3-PHENYLPYRUVIC 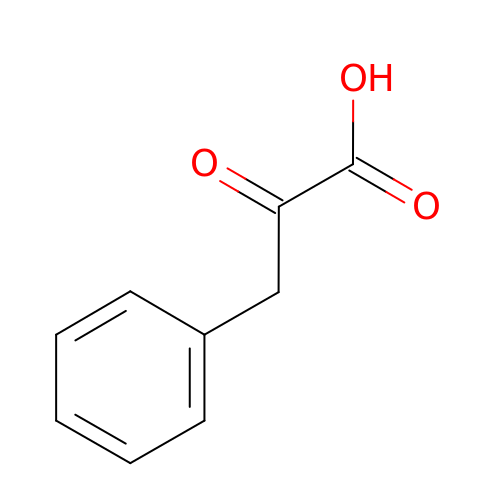ACID | C9 H8 O3 | BTNMPGBKDVTSJY-UHFFFAOYSA-N> MDKSSIANK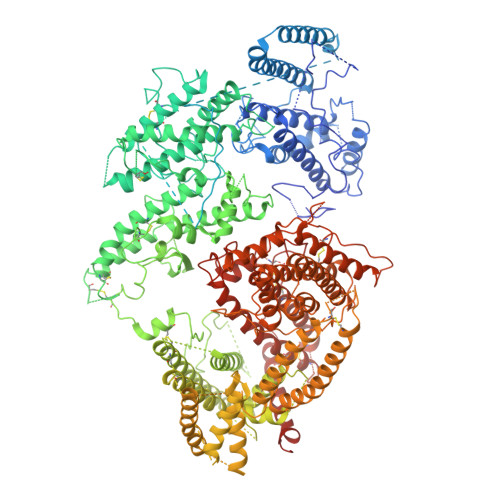IEAYLGAKSDDSKIDQSLKADPSEVQYYGSGGDGYYLRKNICKITVNHSDSGTNDPCDRIPPPYGDNDQWKCAIILSKVSEKPENVFVPPRRQRMCINNLEKLNVDKIRDKHAFLADVLLTARNEGERIVQNHPDTNSSNVCNALERSFADIADIIRGTDLWKGTNSNLEQNLKQMFAKIRENDKVLQDKYPKDQNYRKLREDWWNANRQKVWEVITCGARSNDLLIKRGWRTSGKSNGDNKLELCRKCGHYEEKVPTKLDYVPQFLRWLTEWIEDFYREKQNLIDDMERHREECTSEDHKSKEGTSYCSTCKDKCKKYCECVKKWKSEWENQKNKYTELYQQNKNETSQKNTSRYDDYVKDFFKKLEANYSSLENYIKGDPYFAEYATKLSFILNSSDANNPSEKIQKNNDEVCNCNESGIASVEQEQISDPSSNKTCITHSSIKANKKKVCKHVKLGVRENDKDLRVCVIEHTSLSGVENCCCQDFLRILQENCSDNKSGSSSNGSCNNKNQEACEKNLEKVLASLTNCYKCDKCKSEQSKKNNKNWIWKKSSGKEGGLQKEYANTIGLPPRTQSLCLVVCLDEKGKKTQELKNIRTNSELLKEWIIAAFHEGKNLKPSHEKKNDDNGKKLCKALEYSFADYGDLIKGTSIWDNEYTKDLELNLQKIFGKLFRKYIKKNNTAEQDTSYSSLDELRESWWNTNKKYIWLAMKHGAGMNSTTCCGDGSVTGSGSSCDDIPTIDLIPQYLRFLQEWVEHFCKQRQEKVKPVIENCKSCKESGGTCNGECKTECKNKCEVYKKFIEDCKGGDGTAGSSWVKRWDQIYKRYSKYIEDAKRNRKAGTKNCGPSSTTNAAENKCVQSDIDSFFKHLIDIGLTTPSSYLSIVLDDNICGADKAPWTTYTTYTTTEKCNKETDKSKLQQCNTAVVVNVPSPLGNTPHGYKYACQCKIPTNEETCDDRKEYMNQWSCGSARTMKRGYKNDNYELCKYNGVDVKPTTVRSNSSKLDDKDVTFFNLFEQWNKEIQYQIEQYMTNTKISCNNEKNVLSRVSDEAAQPKFSDNERDRNSITHEDKNCKEKCKCYSLWIEKINDQWDKQKDNYNKFQRKQIYDANKGSQNKKVVSLSNFLFFSCWEEYIQKYFNGDWSKIKNIGSDTFEFLIKKCGNDSGDGETIFSEKLNNAEKKCKENESTNNKMKSSETSCDCSEPIYIRGCQPKIYDGKIFPGKGGEKQWICKDTIIHGDTNGACIPPRTQNLCVGELWDKRYGGRSNIKNDTKESLKQKIKNAIQKETELLYEYHDKGTAIISRNPMKGQKEKEEKNNDSNGLPKGFCHAVQRSFIDYKNMILGTSVNIYEYIGKLQEDIKKIIEKGTTKQNGKTVGSGAENVNAWWKGIEGEMWDAVRCAITKINKKQKKNGTFSIDECGIFPPTGNDEDQSVSWFKEWSEQFCIERLQYEKNIRDACTNNGQGDKIQGDCKRKCEEYKKYISEKKQEWDKQKTKYENKYVGKSASDLLKENYPECISANFDFIFNDNIEYKTYYPYGDYSSICSCEQVKYYEYNNAEKKNNKSLCHEKGNDRTWSKKYIKKLENGRTLEGVYVPPRRQQLCLYELFPIIIKNKNDITNAKKELLETLQIVAEREAYYLWKQYHAHNDTTYLAHKKACCAIRGSFYDLEDIIKGNDLVHDEYTKYIDSKLNEIFDSSNKNDIETKRARTDWWENEAIAVPNITGANKSDPKTIRQLVWDAMQSGVRKAIDEEKEKKKPNENFPPCMGVQHIGIAKPQFIRWLEEWTNEFCEKYTKYFEDMKSNCNLRKGADDCDDNSNIECKKACANYTNWLNPKRIEWNGMSNYYNKIYRKSNKESEDGKDYSMIMEPTVIDYLNKRCNGEINGNYICCSCKNIGENSTSGTVNKKLQKKETQCEDNKGPLDLMNKVLNKMDPKYSEHKMKCTEVYLEHVEEQLKEIDNAIKDY>[2x]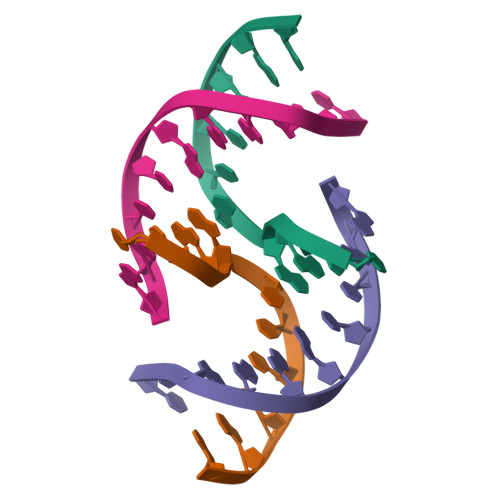CTAACCCTAA;>TTAGGGTTAG[2x]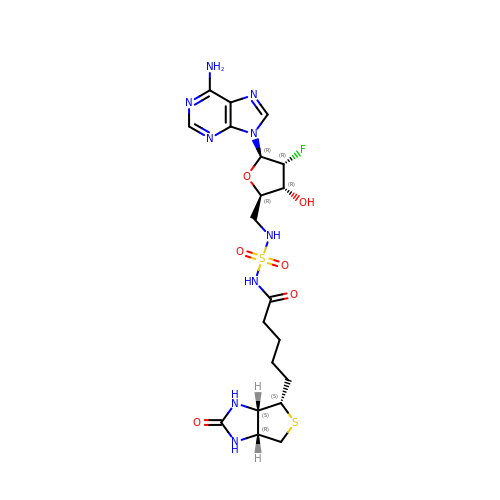2',5'-dideoxy-2'-fluoro-5'-[({5-[(3aS,4S,6aR)-2-oxohexahydro-1H-thieno[3,4-d]imidazol-4-yl]pentanoyl}sulfamoyl)amino]adenosine | C20 H28 F N9 O6 S2 | YGQCUYNQUMQODL-LHWMPIBMSA-N>[2x]MGKIFEDNSLTIGHTPLVRLNRIGNGRILAKVESRNPSFSVKCRIGANMIWDAEKRGVLKPGVELVEPTSGNTGIALAYVAAARGYKLTLTMPETMSIERRKLLKALGANLVLTEGAKGMKGAIQKAEEIVASNPEKYLLLQQFSNPANPEIHEKTTGPEIWEDTDGQVDVFIAGVGTGGTLTGVSRYIKGTKGKTDLISVAVEPTDSPVIAQALAGEEIKPGPHKIQGIGAGFIPANLDLKLVDKVIGITNEEAISTARRLMEEEGILAGISSGAAVAAALKLQEDESFTNKNIVVILPSSGERYLSTALFADLFTEKELQQ;>MVENNALSLVARGCAVAAPCRTKVAEQLLEIGAKAGMAGLAGAAVKDMADRMTSDELEHLITLQM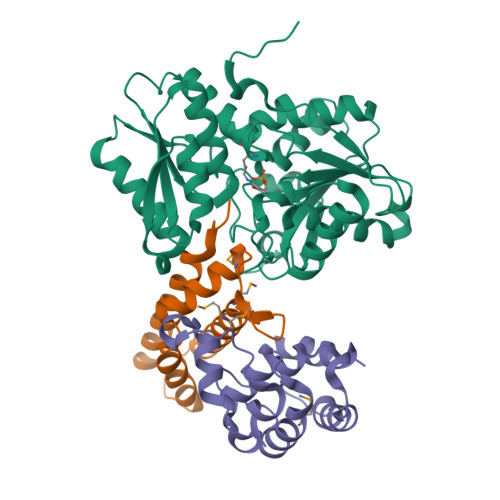MGNDEITTKYLSSLHDKYGSGAASNPNIGKDLTDAEKVELGGSGSGTGTPPPSENDPKQQNEKTVDKLNQKQESAIKKIDNTIKNALKDHDIIGTLKDMDGKPVPKENGGYWDHMQEMQNTLRGLRNHADTLKNVNNPEAQAAYGRATDAINKIESALKGYGI[2x];>MITLRKLIGNINMTKEPEQQSPLELWFERIIDVPLEKLTVEDLCRAIRQNLCIDQLMPRVLEVLTKEPLAGEYYDGELIAALSTIKGEDLKDQKSTFTQIRQLINQLEPSDINDDLRKDILKINQIIVTSLEHHHHHH[2x]> GSKLGEAPADRLKALVDAAVQPVMKANDIPGLAVAISLKGEPHYFSYGLASKEDGRRVTPETLFEIGSVSKTFT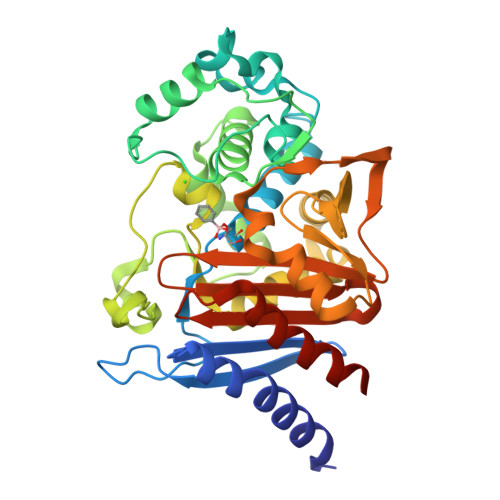ATLAGYALTQDKMRLDDRASQHWPALQGSRFDGISLLDLATYTAGGLPLQFPDSVQKDQAQIRDYYRQWQPTYAPGSQRLYSNPSIGLFGYLAARSLGQPFERLMEQQVFPALGLEQTHLDVPEAALAQYAQGYGKDDRPLRVGPGPLDAEGYGVKTSAADLLRFVDANLHPERLDRPWAQALDATHRGYYKVGDMTQGLGWEAYDWPISLKRLQAGNSTPMALQPHRIARLPAPQALEGQRLLNKTGSTNGFGAYVAFVPGRDLGLVILANRNYPNAERVKIAYAILSGLEQQGKVPLKA>GSHMNDVVDLLPRTEISDKITSELVSKIGDKNWKIRKEGLDEVAGIINDAKFIQPNIGELPTALKGRLNDSNKILVQQTLNILQQLAVAMGPNIKQHVKNLGIPIITVLGDSKNNVRAAALATVNAWAEQTGMKEWLEGEDLSEELKKENPFLRQELLGWLAEKLPTLRSTPTDL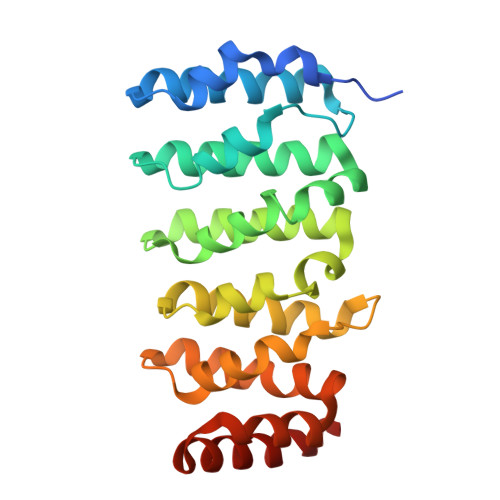ILCVPHLYSCLEDRNGDVRKKAQDALPFFMMHLGYEKMAKATGKLKPTSKDQVLAMLEKAKVNMP[2x]>GPGSELPQMVQQLNSPDQQELQSALRKLSQIASGGNEQIQAVIDAGALPALVQLLSSPNEQILQEALWALSNIASGGNEQIQAVIDAGALPALVQLLSSPNEQILQEALWALRNIASGGNEQIQAVIDAGALPALVQLLSSPNEQILSSALGALSNIASGGNEQIQAVIDAGALPALVQLLSSPNEQILQLALWALSNIASGGNEQIQAVIDAGALPALVQLLSSPNEQILQEALWALSNIASGGNEQIQAVIDAGALPALVQLLSSPNEQILQEALWALSNIASGGNEQKQAVKEAGALEKLEQLQSHENEKI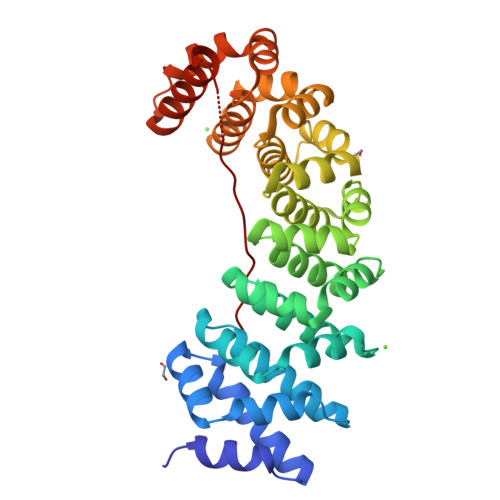QKEAQEALEKLQSHGSGGSGKRKRKLKFKR[6x]> DFDYVVVGAGNAGNVVAARLTEDPDVSVLVLEAGVSDENVLGAEAPLLAPGLVPNSIFDWNYTTTAQAGYNGRSIAYPRGRMLGGSSSVHYMVMMRGSTEDFDRYAAVTGDEGWNWDNIQQFVRKNEMVVPPADNHNTSGEFIPAVHGTNGSVSISLPGFPTPLDDRVLATTQEQSEEFFFNPDMGTGHPLGISWSIASVGNGQRSSSSTAYLRPAQSRPNLSVLINAQVTKLVNSGTTNGLPAFRCVEYAEQEGAPTTTVCAKKEVVLSAGSVGTPILLQLSGIGDENDLSSVGIDTIVNNPSVGRNLSDHLLLPAAFFVNSNQTFDNIFRDSSEFNVDLDQWTNTRTGPLTALIANHLAWLRLPSNSSIFQTFPDPAAGPNSAHWETIFSNQWFHPAIPRPDTGSFMSVTNALISPVARGDIKLATSNPFDKPLINPQYLSTEFDIFTMIQAVKSNLRFLSGQAWADFVIRPFDPRLRDPTDDAAIESYIRDNANTIFHPVGTASMSPRGASWGVVDPDLKVKGVD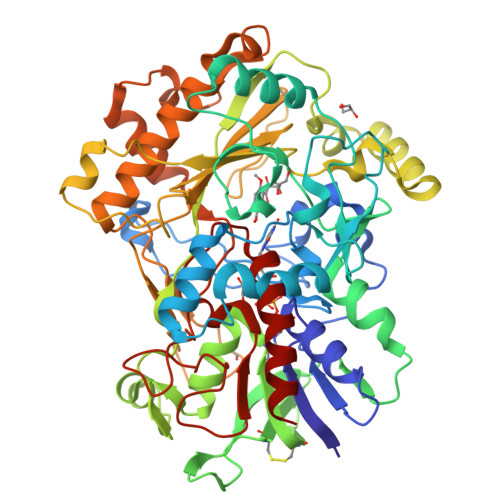GLRIVDGSILPFAPNAHTQGPIYLVGERGADLIKADQ>[2x]PNFSGNWKIIRSENF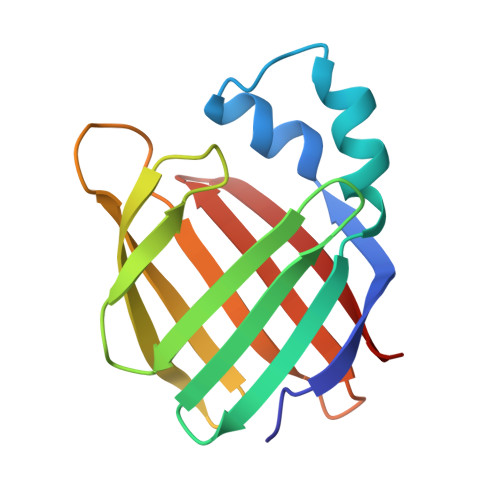EELLKVLGVNVMLRKIAVAAASKPAVEIKQEGDTFYIKTSTTVRTTEINFKVGEEFEEQTVDGRPCKSLVKWESENKMVCEQKLLKGEGPKTSWTMELTNDGELILTMTADDVVCTRVYVRE>[2x]KAMHVAQPAVVLASSRGIASFVCEYASPGKATEVRVTVLRQADSQVTEVCAATY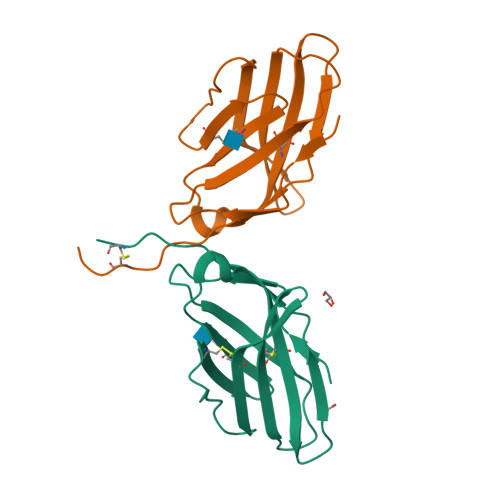MMGNELTFLDDSICTGTSSGNQVNLTIQGLRAMDTGLYICKVELMYPPPYYLGIGNGTQIYVIDPEPCPDSDLVPR> GPGKTDSSFIMDSDPRRCMRHHYVDSISHPLYKCSSKMVLLARCEGHCSQASRSEPLVSFSTVLKQPFRSSCHCCRPQTSKLKALRLRCSGGMRLTATYRYILSCHCEECNSGTETSQVAPA;> DTGERRCDPIRISMCQNLGYNVTKMPNLVGHELQTDAELQLTTFTPLIQYGCSS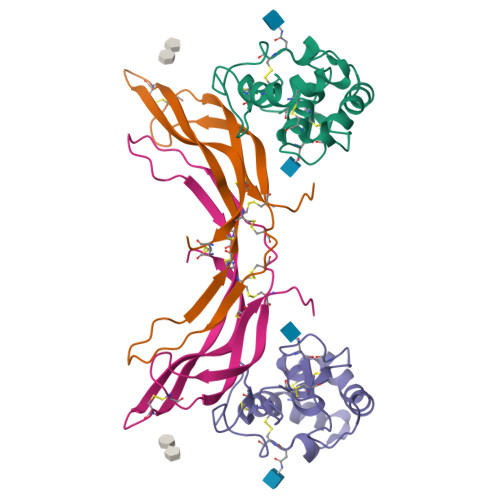QLQFFLCSVYVPMCTEKINIPIGPCGGMCLSVKRRCEPVLKEFGFAWPESLNCSKFPPQNDHNHMCMEGPGDEEVPLPHKTPIQPGEGTLEVLFQ> MWQRLRFDRLSSSVRRTNLNPLKPCAALTEQRAELRNLHQYPTARHKSLVKDRLRFARNWWLTGGNNYELVHEVGHEREATECFAEYAQDSSRDVYLMSTNRLSDLPPGDRLKAIVGLMRSRWEVKDANRGYDKAKLLLQALECFSEMKASG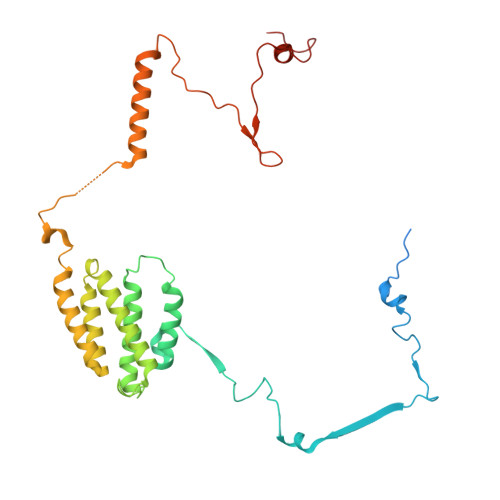QIGDFNSLPEPDQDTFLQYVEGCSRFAQACSHSHPDAVRVLLRAAQICEEMRCVEKRDEMIQVTEAAANRMDRAYAFSRPHDTLRAAPPSLHENEDCVRLKNTEELRRRFGNTAPHVLEKPKRVDCLRIHRNRPLLLHPMKDNNKLLELSKLPARPEFDSWTSHQT>[2x]GSHMRGEFYQQLTNDLETARAEGLFKEERIITSAQQADITVADGSHVINFCANNYLGLANHPDLIAAAKAGMDSHGFGMASVRFICGTQDSHKELEQKLAAFLGMED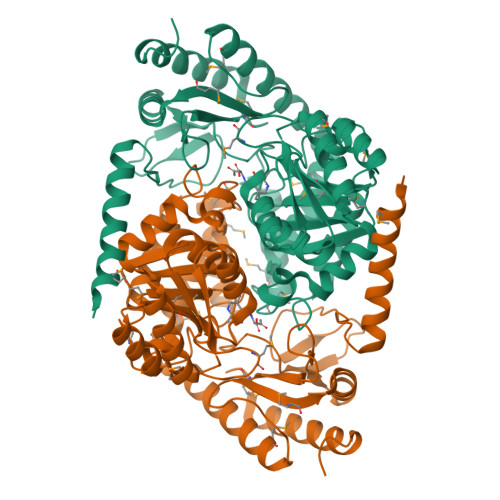AILYSSCFDANGGLFETLLGAEDAIISDALNHASIIDGVRLCKAKRYRYANNDMQELEARLKEAREAGARHVLIATDGVFSMDGVIANLKGVCDLADKYDALVMVDDSHAVGFVGENGRGSHEYCDVMGRVDIITGTLGKALGGASGGYTAARKEVVEWLRQRSRPYLFSNSLAPAIVAASIKVLEMVEAGSELRDRLWANARQFREQMSAAGFTLAGADHAIIPVMLGDAVVAQKFARELQKEGIYVTGFFYPVVPKGQARIRTQMSAAHTPEQITRAVEAFTRIGKQLGVIA>MDIDNYRVKPGKRVKLSDWATNDDAGLSKEEGQAQTAKLAGELAEWQERLYAEGKQSLLLILQARDAAGKDGAVKKVIGAFNPAGVQITSFKQPSAEELSHDFLWRIHQKAPAKGYVGVFNRSQYEDVLVTRVYDMIDDKTAKRRLEHIRHFEELLTDNA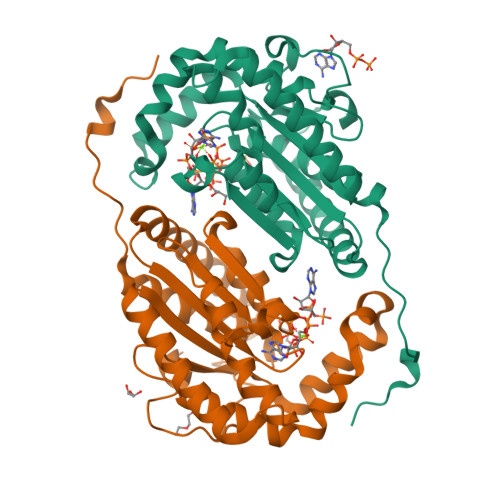TRIVKVYLHISPEEQKERLQARLDNPGKHWKFNPGDLKDRSNWDKFNDVYEDALTTSTDDAPWYVVPADRKWYRDLVLSHILLGALKDMNPQFPAIDYDPSKVVIH[4x]> MAKVHVTDVVLRDGHQSLIATRMRTDDMLPICSKLDAVGYWSLEAWGGATFDACVRYLREDPWERLKKLRKALPNSRLQMLLRG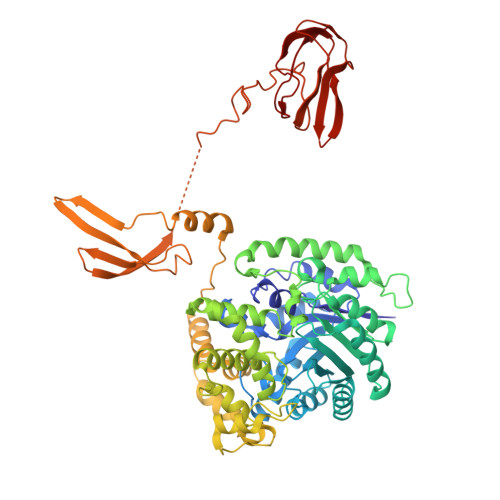QNLLGYRHYSDDVVRAFVQKSADNGIDVFRIFDAMNDLRNLKVSIESVKAVGKHAEGTISYTTSPVHDIPYFVNLAKELESFGCDTIAIKDMASLLTPQVTGDLVKALREAVSLPIHLHAHATSGLASMSIQRAVDNGVAIVDGCISSFAEGASLPATESIVAALKGTEYDTGLDIGLLQEISAYFREVRKKYWQFESEFTGVDTRVLVNQVPGGMISNLSNQLKEQGALDRMDAVLDEIPRVREDLGYPPLVTPTSQIVGTQAVLNVMTGARYKSVTNEVKNYLLGHYGKAPSTVNPDVRNLAVGNAQVIECRPADLLTAEMEKLRNEVEGLAASAADVLTYAMFPDLAKTFLQERNAGSLKPEPLLDKEAVTSRESHSRFAPTEFNVTLHGETFHIKLTGSGHHGEEQRPFYVSVDGVTEEVVVEILNEIEVSGGGQSSGEAKRKASSAASSGRPRPTHAGCVTTAMPGTIVDVKVNVGDKVSAGDAVLVIEAMKMENEIQASKSGVVVAINVKKGDSVTPDEALLEIQPD>MTSITPVTLANCEDEPIHVPGAIQPHGALVTLRADGMVLAASENIQALLGFVASPGSYLTQEQVGPEVLRMLEEGLTGNGPWSNSVETRIGEHLFDVIGHSYKEVFYLEFEIRTADTLSITSFTLNAQRIIAQVQLHNDTASLLSNVTDELRRMTGYDRVMAYRFRHDDSGEVVAESRREDLESYLGLRYPASDIPAQARRLYIQNPIRLIADVAYTPMRVFPALNPETNESFDLSYSVLRSVSPIHCEYLTNMGVRASMSISIVVGGKLWGLFSCHHMSPKL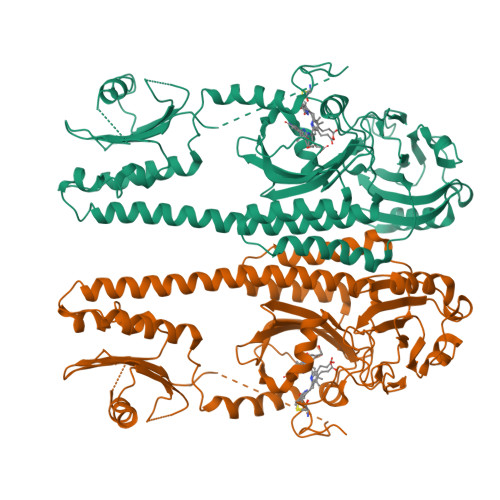IPYPVRMSFQIFSQVCSAIVERLEQGRIAELLRVSTERRLALARRARDADDLFGALAHPDDGIAALIPCDGALVMLGGRTLSIRGDFERQAGNVLQRLQRDPERDIYHTDNWPQPSEDSPDGGDCCGVLAIRFHRQESGWIFWFRHEEVHRIRWGGKPEKLLTIGPSGPRLTPRGSFEAWEEVVRGHSTPWSETDLAIAEKLRLDLMELCLNHALEHHHHHH[2x]> MSQSNRELVVDFLSYKLSQKGYSWSQFSDVEENRTEAPEGTESEMETPSAINGNPSWHLADSPAVNGATGHSSSLDAREVIPMAAVKQALREAGDEWELRYRRAFSDLTSQLHITPGTAYQSFEQVVNELFRDGVNW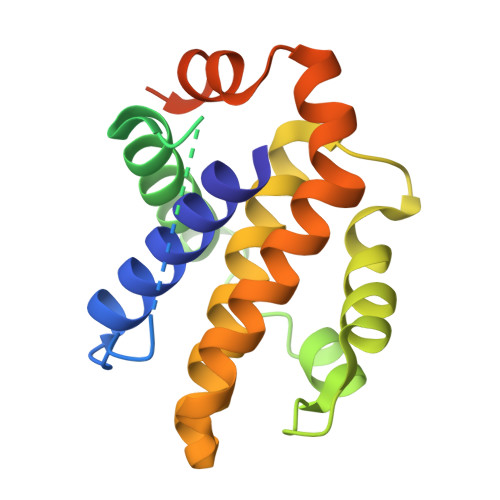GRIVAFFSFGGALCVESVDKEMQVLVSRIAAWMATYLNDHLEPWIQENGGWDTFVELYGNNAAAESRKGQERFNEHHHHHH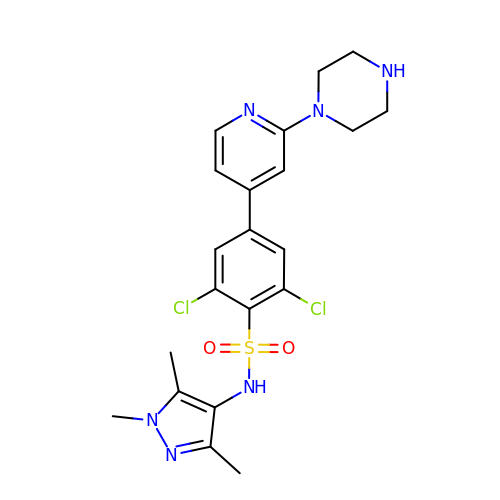2,6-dichloro-4-(2-piperazin-1-ylpyridin-4-yl)-N-(1,3,5-trimethyl-1H-pyrazol-4-yl)benzenesulfonamide | C21 H24 Cl2 N6 O2 S | XMBSZPZJLPTFMV-UHFFFAOYSA-N>[2x]MNYFVGNSLGVNLTGIEKAIINRLNLFKEMGRPAQCVFLSWNRYLYRNAQNYITSSDYINMYDFFQEATYLERNEPFDWLSYWTDECHYTLKHVENSHDFRIYDQERFLMYAHFQDPKYRILDYVNHFDSQRRKVKRDFYDVRGFLSCSRILVDKQQTLCEFFYNPEGDTKLEKYFSYKDGKPEVQKIIVYYANKQYFFNNETELGAFFIKQLYQHGDLFFSDRNVYTAPIFNLTPESIPVVAVLHSTHIKNIDALDSSPFKNVYKAMFENLSRYRAIIVSTEQQKLDVEKRINHTIPVVNIPVGYSETIDTPVQTLDQRSVKLISVARYSPEKQLHQQIELIKRLVSYVPKIELHMYGFGSESKKLNELIQKYGLENHVYLRGFLSNLDQEYSDAYLSLITSNMEGFSLALLESLAHGVPVISYDIKYGPNELITSDFNGYLITKNDEDALFDKVKYVIDHPEVQQRLSKGSLAKAQQYSKASLIKQWDQFVRLILEHHHHHH

Two glycosyltransferases (GTases), SdgB and SdgA, are responsible for the glycosylation of S. aureus SDR proteins such as ClfA and ClfB. SdgB first appends N-acetyl­glucosamine (GlcNAc) moieties onto serine residues (O-glycosylation) within the SDR domain using uridine diphos­phate N-acetylglucosamine (UDP-GlcNAc) as a donor substrate. The subsequent addition of GlcNAc to the glycoproteins is catalyzed by the second enzyme, SdgA, yielding glycosylated SDR proteins in which each SD repeat is decorated with GlcNAc disaccharide moieties. The glycosylation of SDR proteins mediated by SdgA and SdgB protects SDR proteins from degradation by host proteases, thereby circumventing innate immune attack.

Despite the biological significance of these two glycosyltransferases involved in pathogenicity and avoidance of the host innate immune response, their structures and the molecular basis of their activity have not been investigated. This study reports the crystal structures of SdgB and SdgA from S. aureus as well as multiple structures of SdgB in complex with its substrates (for example UDP, N-acetylglucosamine or SDR peptides), products (glycosylated SDR peptides) or phosphate ions. Altogether, the extensive snapshots of SdgB complexes in multiple states provided a mechanistic insight into how SdgB recognizes and glycosylates the clustered serine residues in the SDR proteins.>MAFKRHIDRLPIIPADAKKHNVTCHFCIVGCGYHAYTWPINKQGGTDPQNNIFGVDLSEQQQAESDAWYSPSMYNVVKQDGRDVHVVIKPD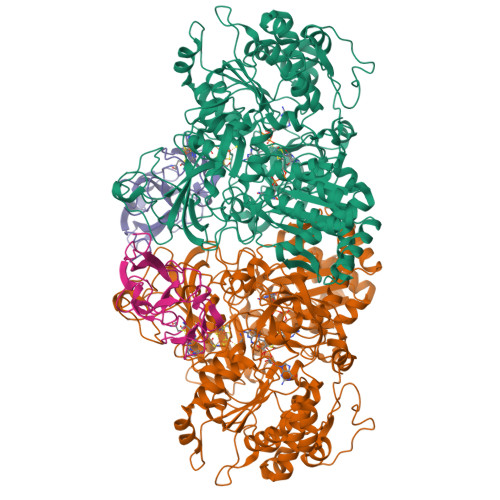HECVVNSGLGSVRGARMAETSFSEARNTQQQRLTDPLVWRYGQMQPTSWDDALDLVARVTAKIVKEKGEDALIVSAFDHGGAGGGYENTWGTGKLYFEAMKVKNIRIHNRPAYNSEVHGTRDMGVGELNNCYEDAELADTIVAVGTNALETQTNYFLNHWIPNLRGESLGKKKELMPEEPHEAGRIIIVDPRRTVTVNACEQTAGADNVLHLAINSGTDLALFNALFTYIADKGWVDRDFIDKSTLREGTARPPLYPARGVSEANPGHLSSFEDAVEGCRMSIEEAAEITGLDAAQIIKAAEWIGMPKEGGKRRRVMFGYEKGLIWGNDNYRTNGALVNLALATGNIGRPGGGVVRLGGHQEGYVRPSDAHVGRPAAYVDQLLIGGQGGVHHIWGCDHYKTTLNAHEFKRVYKKRTDMVKDAMSAAPYGDREAMVNAIVDAINQGGLFAVNVDIIPTKIGEACHVILPAATSGEMNLTSMNGERRMRLTERYMDPPGQSMPDCLIAARLANTMERVLTEMGDVGYAAQFKGFDWQTEEDAFMDGYNKNAHGGEFVTYERLSAMGTNGFQEPATGFTDGKIEGTQRLYTDGVFSTDDGKARFMDAPWRGLQAPGKQQQKDSHKYLINNGRANVVWQSAYLDQENDFVMDRFPYPFIEMNPEDMAEAGLKEGDLVEIYNDAGATQAMAYPTPTARRGETFMLFGFPTGVQGNVTSAGTNELIIPNYKQTWGNIRKISDAPRNVAHLSFKSKEYQSA[4x];>[4x]MSRCQNMVDIGRRQFLRGGALAAAGATAAVFGVGAPQARAATAAAGVEYPANRLANISELTLNEPLDVAYPDEDAAGVLLKLGTRVEGGVGPDGDIVGFSTICPHKGFPLSYSADNKTFNCPGHFSVFDPEKGGQQVWGQATQNLPQYVLRVADNGDIFAEGVDELIYGRLSNVL>[3x]MPAL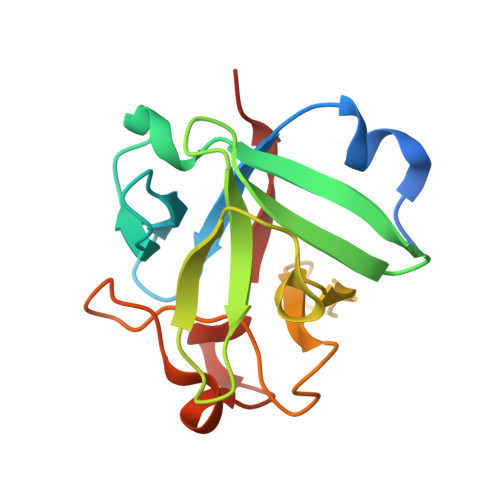PEDGGSGAFPPGHFKEPKRLYCKNGGFFLRIHPDGRVDGVREKSDPHIKLQLQAEERGVVSIKGVIANRYLAMKEDGRLLASKIVTDECFFFERLESNNYNTYRSRKYTSWYVALKRTGQYKLGPKTGPGQKAILFLPMSAKS> MQNSQDFSITELSLPKGGGAITGMGEALTPTGPDGMAALSLPLPISAGRGYAPAFTLNYNSGAGNSPFGLGWDCNVMTIRRRTHFGVPHYDETDTFLGPEGEVLVVADQPRDESTLQGINLGATFTVTGYRSRLESHFSRLEYWQPKTTGKTDFWLIYSPDGQVHLLGKSPQARISNPSQTTQTAQWLLEASVSSRGEQIYYQYRAEDDTGCEADEITHHLQATAQRYLHIVYYGNRTASETLPGLDGSAPSQADWLFYLVFDYGERSNNLKTPPAFSTTGSWLCRQDRFSRYEYGFEIRTRRLCRQVLMYHHLQALDSKITEHNGPTLVSRLILNYDESAIASTLVFVRRVGHEQDGNVVTLPPLELAYQDFSPRHHAHWQPMDVLANFNAIQRWQLVDLKGEGLPGLLYQDKGAWWYRSAQRLGEIGSDAVTWEKMQPLSVIPSLQSNASLVDINGDGQLDWVITGPGLRGYHSQRPDGSWTRFTPLNALPVEYTHPRAQLADLMGAGLSDLVLIGPKSVRLYANTRDGFAKGKDVVQSGDITLPVPGADPRKLVAFSDVLGSGQAHLVEVSATKVTCWPNLGRGRFGQPITLPGFSQPATEFNPAQVYLADLDGSGPTDLIYVHTNRLDIFLNKSGNGFAEPVTLRFPEGLRFDHTCQLQMADVQGLGVASLILSVPHMSPHHWRCDLTNMKPWLLNEMNNNMGVHHTLRYRSSSQFWLDEKAAALTTGQTPVCYLPFPIHTLWQTETEDEISGNKLVTTLRYARGAWDGREREFRGFGYVEQTDSHQLAQGNAPERTPPALTKNWYATGLPVIDNALSTEYWRDDQAFAGFSPRFTTWQDNKDVPLTPEDDNSRYWFNRALKGQLLRSELYGLDDSTNKHVPYTVTEFRSQVRRLQHTDSRYPVLWSSVVESRNYHYERIASDPQCSQNITLSSDRFGQPLKQLSVQYPRRQQPAINLYPDTLPDKLLANSYDDQQRQLRLTYQQSSWHHLTNNTVRVLGLPDSTRSDIFTYGAENVPAGGLNLELLSDKNSLIADDKPREYLGQQKTAYTDGQNTTPLQTPTRQALIAFTETTVFNQSTLSAFNGSIPSDKLSTTLEQAGYQQTNYLFPRTGEDKVWVAHHGYTDYGTAAQFWRPQKQSNTQLTGKITLIWDA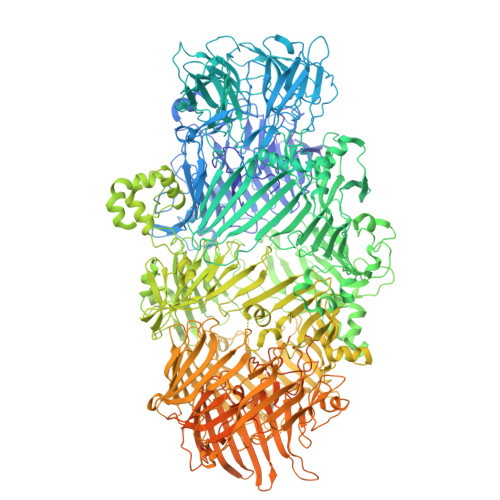NYCVVVQTRDAAGLTTSAKYDWRFLTPVQLTDINDNQHLITLDALGRPITLRFWGTENGKMTGYSSPEKASFSPPSDVNAAIELKKPLPVAQCQVYAPESWMPVLSQKTFNRLAEQDWQKLYNARIITEDGRICTLAYRRWVQSQKAIPQLISLLNNGPRLPPHSLTLTTDRYDHDPEQQIRQQVVFSDGFGRLLQAAARHEAGMARQRNEDGSLIINVQHTENRWAVTGRTEYDNKGQPIRTYQPYFLNDWRYVSNDSARQEKEAYADTHVYDPIGREIKVITAKGWFRRTLFTPWFTVNEDENDTAAEVKKVKMMKNIDPKLYQKTPTVSVYDNRGLIIRNIDFHRTTANGDPDTRITRHQYDIHGHLNQSIDPRLYEAKQTNNTIKPNFLWQYDLTGNPLCTESIDAGRTVTLNDIEGRPLLTVTATGVIQTRQYETSSLPGRLLSVAEQTPEEKTSRITERLIWAGNTEAEKDHNLAGQCVRHYDTAGVTRLESLSLTGTVLSQSSQLLIDTQEANWTGDNETVWQNMLADDIYTTLSTFDATGALLTQTDAKGNIQRLAYDVAGQLNGSWLTLKGQTEQVIIKSLTYSAAGQKLREEHGNDVITEYSYEPETQRLIGIKTRRPSDTKVLQDLRYEYDPVGNVISIRNDAEATRFWHNQKVMPENTYTYDSLYQLISATGREMANIGQQSHQFPSPALPSDNNTYTNYTRTYTYDRGGNLTKIQHSSPATQNNYTTNITVSNRSNRAVLSTLTEDPAQVDALFDAGGHQNTLISGQNLNWNTRGELQQVTLVKRDKGANDDREWYRYSGDGRRMLKINEQQASNNAQTQRVTYLPNLELRLTQNSTATTEDLQVITVGEAGRAQVRVLHWESGKPEDIDNNQLRYSYDNLIGSSQLELDSEGQIISEEEYYPYGGTALWAARNQTEASYKTIRYSGKERDATGLYYYGYRYYQPWIGRWLSSAPAGTIDGLNLYRMVRNNPVTLLDPDGLMPTIAERIAALKKNKVTDSAPSPANATNVAINIRPPVAPKPSLPKASTSSQPTTHPIGAANIKPTTSGSSIVAPLSPVGNKSTSEISLPESAQSSSSSTTSTNLQKKSFTLYRADNRSFEEMQSKFPEGFKAWTPLDTKMARQFASIFIGQKDTSNLPKETVKNISTWGAKPKLKDLSNYIKYTKDKSTVWVSTAINTEAGGQSSGAPLHKIDMDLYEFAIDGQKLNPLPEGRTKNMVPSLLLDTPQIETSSIIALNHGPVNDAEISFLTTIPLKNVKPHKR> MHHHHHHGENLYFQGSAAHHRQNTAGRRKVQVSYVIRDEVEKYNRNGVNALQLDPALNRLFTAGRDSIIRIWSVNQHKQDPYIASMEHHTDWVNDIVLCCNGKTLISASSDTTVKVWNAHKGFCMSTLRTHKDYVKALAYAKDKELVASAGLDRQIFLWDVNTLTALTASNNTVTTSSLSGNKDSIYSLAMNQLGTIIVSGSTEKVLRVWDPRTCAKLMKLKGHTDNVKALLLNRDGTQCLSGSSDGTIRLWSLGQQRCIATYRVHDEGVWALQVNDAFTHVYSGGRDRKIYCTDLRNPDIRVLICEEKAPVLKMELDRSADPPPAIWVATTKSTVNKWTLKGIHNFRASGDYDND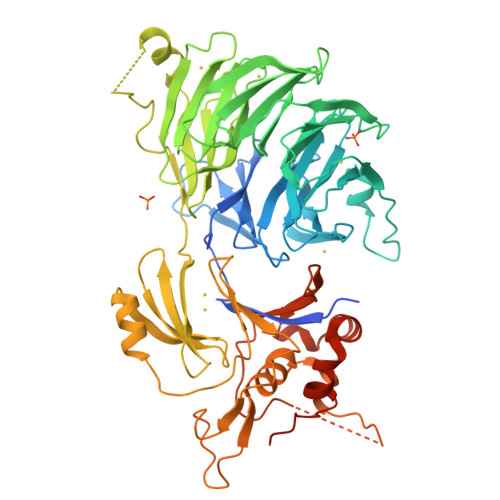CTNPITPLCTQPDQVIKGGASIIQCHILNDKRHILTKDTNNNVAYWDVLKACKVEDLGKVDFEDEIKKRFKMVYVPNWFSVDLKTGMLTITLDESDCFAAWVSAKDAGFSSPDGSDPKLNLGGLLLQALLEYWPRTHVNPMDEEENEVNHVNGEQENRVQKGNGYFQVPPHTPVIFGEAGGRTLFRLLCRDSGGETESMLLNETVPQWVIDITVDKNMPKFNKIPFYLQPHASSGAKTLGNS> KVEEVQT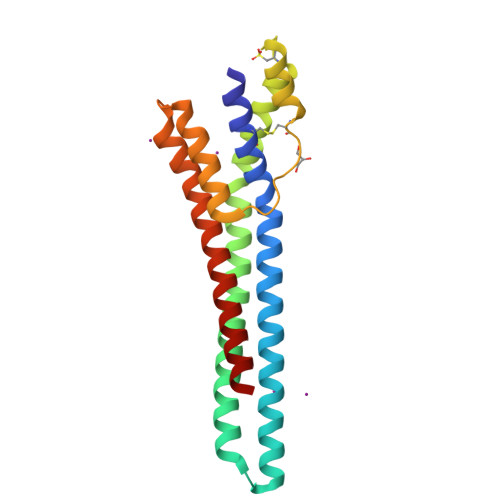MCDVARQLRALETASQSAVAAVVSSAREASEAKERAEKAVERAKSKKRGVDTATEAAARAAAAAQRAETVVSDARKHAADLTAASKDAIETTDESLRLLATCEADEPIRTAAKKCTGAAAEVTSKSLESAFDALAELLPDGADDIREHGAVFVKGLKSLEDDVRTAGEAKYEAEKAE>MSQPTAGAPAAPKARSCPFLPPDGIADIRAAAPVTRATFTSGHEAWLVTGYEQVRAVLRDPSFSVGVPHALHTQDGVVTQKPGRGSLLWQDAPEHTDDRKLLAKEFTVRRMQALRPNIQRIVDEHLDAIEARGGPVDLVKTFANPVPSMVISDLFGVPAERRAEFQEIAEAMMRVDQDAAATEAAGMRLGGLLYQLVQERRANPGDDLISAL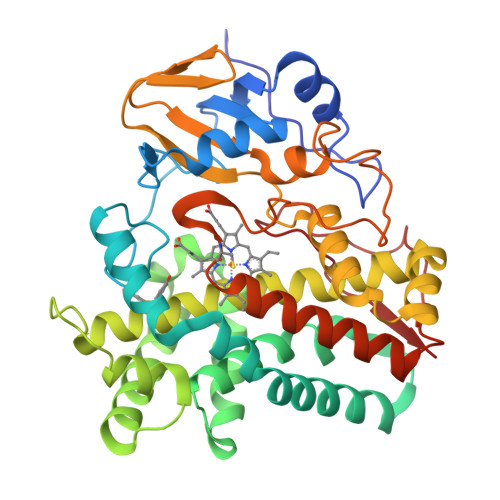ITTEDPDGVIDDMFLMNAAGTLLIAAHDTTACMIGLGTALLLDRPDQLALLQKDPSLIGNAVEELLRYLTIGQFGAERVATQDGEIGGVRIAKGEQVVTHLLSADFDPAFVEDPERFDITRRPAPHLAFGFGAHQCIGQQLARIELQIVFGTLFRRFPTLRLAKPVEELRFRNDMVFYGVHELPVTW[4x]TRICOSANOIC 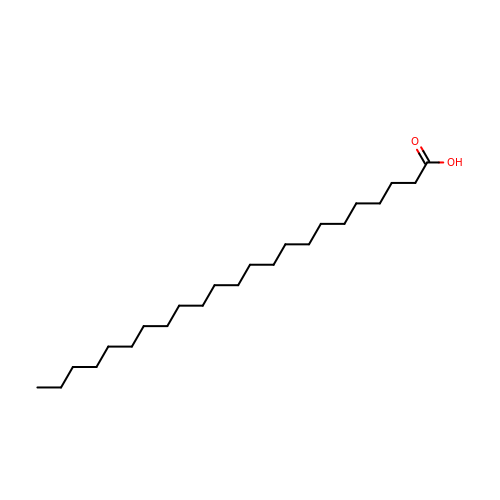ACID | C23 H46 O2 | XEZVDURJDFGERA-UHFFFAOYSA-N> MKVYQTNEIKNIALLGSSGSGKTTLVEAMLFESGVIKRRGSVAAKNTVSDYFPVEQEYGYSVFSTVLHVEWNNKKLNIIDCPGSDDFVGSTVTALNVTDTAIILLNGQYGVEVGTQNHFRYTEKLNKPVIFLVNQLDNEKCDYDNILEQLKEAYGSKVVPIQYPIATGPGFNALIDVLLMKKYSWKPEGGAPVIEDIPAEEMDKAMEMHKALVEAAAENDEGLMEKFFEQDSLTEDEMREGIRKGLIARGMFPVFCVCGGKDMGVRRLMEFLGNVVPFVSEMPKVENTDGKEVAPDVNGPESLYFFK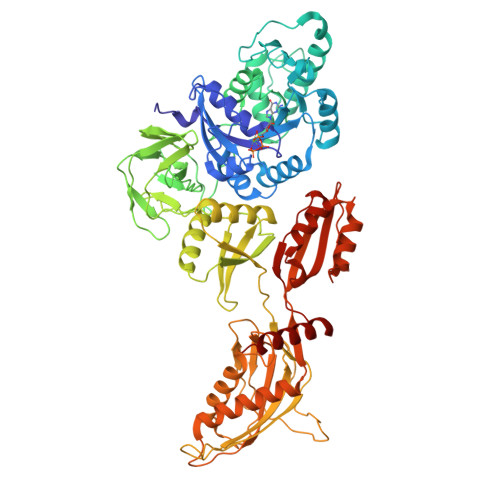TSVEPHIGEVSYFKVMSGKVREGDDLLNADRGSKERIAQIYVVAGGNRVKVEELQAGDIGAAVKLKDVKTGNTLNGKDCDYKFNFIKYPNSKYSRAIKPVNEADVEKMMTILNRMREEDPTWVIEQSKELKQTLVHGQGEFHLRTLKWRLENNEKLQVKFEEPKIPYRETITKAARADYRHKKQSGGAGQFGEVHLIVEPYKEGMPVPDTYKFNGQEFKITVRGTEEIPLEWGGKLVFINSIVGGSIDARFLPAIMKGIMSRLEQGPLTGSYARDVRVIVYDGKMHPVDSNEISFMLAGRNAFSEAFKNAGPKILEPIYDVEVFVPSDRMGDVMGDLQGRRAMIMGMSSEKGFEKLVAKVPLKEMSSYSTALSSLTGGRASFIMKFASYELVPTDVQDKLIKDFEAKQTEE>[3x]GGLEKDFLPLYFGWFLTKKSSETLRKAGQVFLEELGNHKAFKKELRHFISGDEPKEKLELVSYFGKRPPGVLHCTTKFCDYGKAAGAEEYAQQEVVKRSYGKAFKLSISALFVTPKTAGAQVVLTDQELQLWPSDLDKPSASEGLPPGSRAHVTLGCAADVQPVQTGLDLLDILQQVKGGSQGEAVGELPRGKLYSLGKGRWMLSLTKKMEVKAIFTGYYG

2′,3′-cyclic nucleotide 3′-phosphodiesterase (CNPase), one of the proteins predominantly expressed in the myelin sheath, represents 4% of total protein in central nervous system myelin. CNPase belongs to the 2H phosphoesterase superfamily, which is characterized by the presence of two conserved HxT/Sx motifs (x denoting a hydrophobic residue) in the active site. CNPase contains an N-terminal domain very distantly related to P-loop containing nucleoside triphosphate hydrolases and a C-terminal phosphodiesterase domain. We solved the crystal structure of the C-terminal catalytic phosphodiesterase domain of mouse CNPase in the presence of active-site ligands, including reaction products.

In CNPase crystallized in concentrated ammonium sulphate, two sulphate molecules are located in the vicinity of the catalytic site. The active-site sulphate mimics the substrate phosphate group and interacts with all 4 conserved residues of the two HxTx motifs and the two central water molecules in the catalytic site through H-bonds, being also in contact with the backbone carbonyl of Pro320 and bulk solvent. The second sulphate stabilizes the long α6-β5 loop. Arg307, between the two sulphate binding sites, adopts a different conformation in the sulphate complex, turning away from the active site. The significance of the α6-β5 loop is not known, but the detection of a sulphate-binding site and the different conformations seen for the loop suggest it could be relevant in CNPase function.> MDPGLKPSSLWTHKIIDSIIANRSLSAVQNFRKQPLANKLTALEDAIVQPRKDTTPETVAAILQELVAMGALQPNEVGPMFSDLMIRVHKYNSTNVQNNLSVLLGDIRAAQSEAIRSTNVGELSNQVVLNDFLSREPAVVPQGQHNYEAFKQTLRLMVNEAPNVTLFKSGPDTLMQVNIRGVNTVNLNSAFKNLKNFWGVQLDTEIVPGSISSKLSSNTRVLLLFLAPFTNDSTFTPDTFISQIMRLYRETVAASIEQPQETELEVAETIRELGGDVEDIGRTMAFLLKNKEEIVSNPRTLSPRQLNVLRYVQESLQDRIDRNGEEPEDALRNLVFSFAPSYFEANGPFIRRLISYLEVALINSPNYFREIYSNKYWTPPASFWTQNYGDFHLEREAEAERRAASEAGYGDFEEGDFALPDNLGEGSDLAWDDFNTAMSPSVPPTPSVRSAPASLSYGRTSPSSVSSLTASDRNIGATLARAVIPPAAAAIGSAAGEALYPSLGQYLAPAASLAATRLLNLTRARRQRLKRDSLARHRRITEVRGVYPK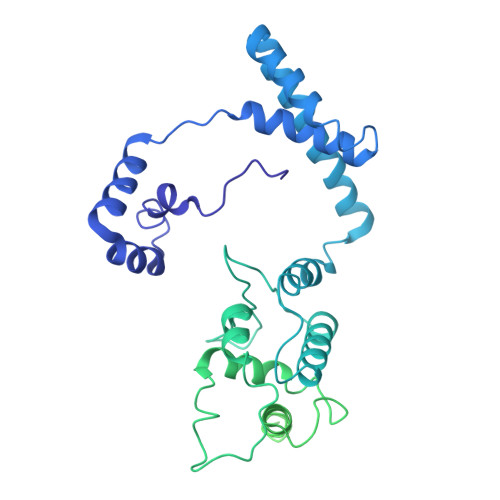AAPTRSSSSSSVSSTPTVFEPLPGAFSVINPLMRPEGDRDVSGTGIVNPFSHLKPRNGLQ[[(2R,3S,4R,5R)-5-(6-aminopurin-9-yl)-3,4-bis(oxidanyl)oxolan-2-yl]methoxy-oxidanyl-phosphoryl] [(2R,3S,4S)-5-azanyl-2,3,4-tris(oxidanyl)pentyl] 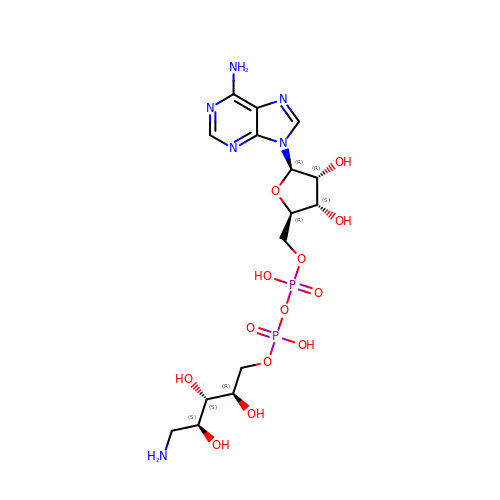hydrogen phosphate | C15 H26 N6 O13 P2 | JFHZDRWPWXRIBP-AOOZFPJJSA-N>[2x]GAHMSVIKPEMKIKLCMRGTVNGHN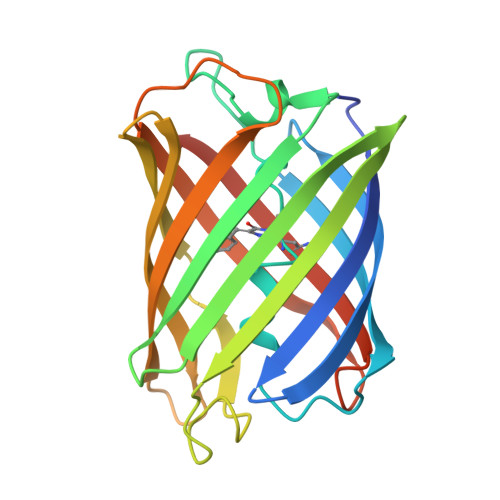FVIEGEGKGNPYEGTQILDLNVTEGAPLPFAYDILTTVFQYGNRAFTKYPADIQDYFKQTFPEGYHWERSMTYEDQGICTATSNISMRGDCFFYDIRFDGTNFPPNGPVMQKKTLKWEPSTEKMYVEDGVLKGDVNMRLLLEGGGHYRCDFKTTYKAKKEVRLPDAHKIDHRIEILKHDKDYNKVKLYENAVARYSMLPSQAK>GSHMDLRAELLKALLKAVEEFLKAAEEAIKELLELLKKALEVLKKLDPKSKGVEALVKGAKGAAKGIEAAMKIAKAVLEVAKIKVEKAIAGEVDPEEALRALRAALEIAFAAFELACEVLKKTLEAIKAVADDKYTAAILAGDNPAAQQKALAETNALCTDSLIAVEGVEKGLKGAYLALEAIIEALEVAEDEEGLKIVA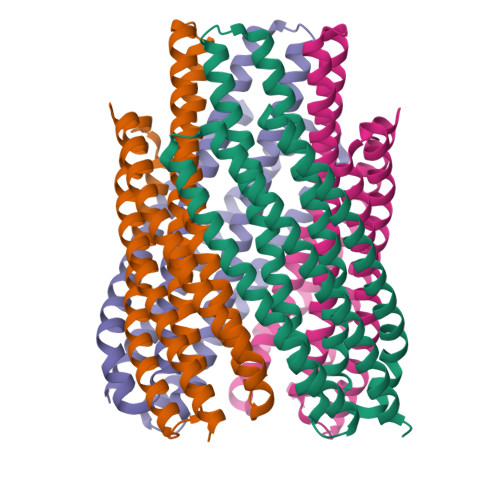KAIKEAIKKAEEAIKKAEEAIKLAKESVEKNLEKLKA[8x]> ELLDPCGYISPESPVVQLHSNFTAVCVLKEKCMDYFHVNANYIVWKTNHFTIPKEQYTIINRTASSVTFTDIASLNIQLTCNILTFGQLEQNVYGITIISGLPPEKPKNLSCIVNEGKKMRCEWDGGRETHLETNFTLKSEWATHKFADCKAKRDTPTSCTVDYSTVYFVNIEVWVEAENALGKVTSDHINFDPVYKVKPNPPHNLS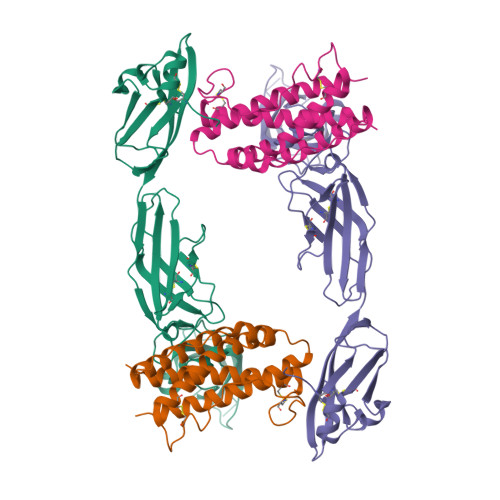VINSEELSSILKLTWTNPSIKSVIILKYNIQYRTKDASTWSQIPPEDTASTRSSFTVQDLKPFTEYVFRIRCMKEDGKGYWSDWSEEASGITYEDR;> LPDAPEFEKDLLIQRLNWMLWVIDECFRDLCYRTGICKGILEPAAIFHLKLPAINDTDHCGLIGFNETSCLKKLADGFFEFEVLFKFLTTEFGKSVINVDVMELLTKTLGWDIQEELNKLTKTHYSPPKFDRGLLGRLQGLKYWVRHFASFYVLSAMEKFAGQAVRVLDSIPDVTPDVHDK> 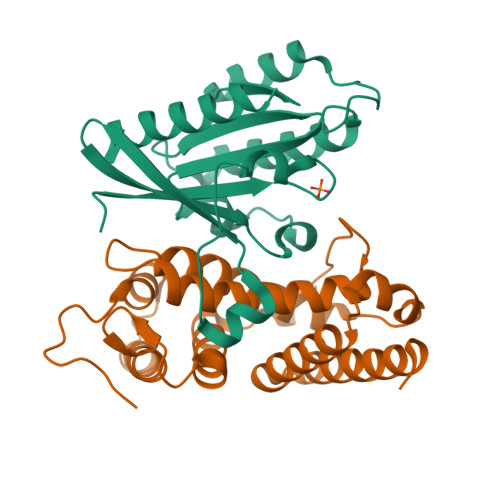GHMPEYDYLFKLLLIGDSGVGKSCLLLRFADDTYTESYISTIGVDFKIRTIELDGKTIKLQIWDTAGQERFRTITSSYYRGAHGIIVVYDVTDQESYANVKQWLQEIDRYASENVNKLLVGNKSDLTTKKVVDNTTAKEFADSLGIPFLETSAKNATNVEQAFMTMAAEIKKRMG;> GHMVTRIENLENAKKLWDNANSMLEKGNISGYLKAANELHKFMKEKNLKEDDLRPELSDKTISPKGYAILQSLWGAASDYSRAAATLTESTVEPGLVSAVNKMSAFFMDCKLSPNERATPDPDFKVGKSKILVGIMQFIKDVADPTSKIWMHNTKALMNHKIAAIQKLERSNNVNDETLESVLSSKGENLSEYLSYK> RSPWGDELLNICMNAKHHKRVPSPE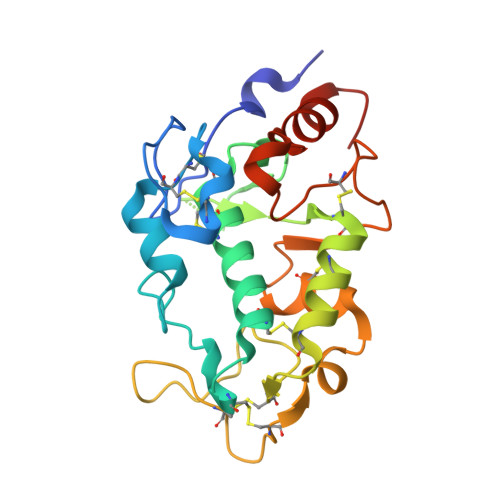DKLYEECIPWKDNACCTLTTSWEAHLDVSPLYNFSLFHCGLLMPGCRKHFIQAICFYECSPNLGPWIQPVGSLGWEVAPSGQGERVVNVPLCQEDCEEWWEDCRMSYTCKSNWRGGWDWSQGKNRCPKGAQCLPFSHYFPTPADLCEKTWSNSFKASPERRNSGRCLQKWFEPAQGNPNVAVARLFASEFLEVLFQ> SFFYDRSTLSSVLQSTSDVSSKFTPSTAKNLQNSILLTPLPSDIVNNSVLPEQERWISFASPTTQKPPYKTKQDWNFIMFSPFTYYKCDLEVTLSKNDRETISSVVRYVPCGAPSDLSDQTMPQTPSLADTRDPHMWVVGQGTTNQISFVIPYTSPLSVLPSVWFNGFSNFDNSSRFGVAPNADFGRLLLQGQGTFSVHYRYKKMRVFCPRPTVFIPWP;> LLSLCKIPTFLGNLDSNKKRIPYFSATNSTPATPLVTYQVTLSCSCMANSMLAAVARNFNQYRGSLNYLFVFTGSAMTKGKFLISYTPPGAGEPKTLDQAMQATYAIWDLGLNSSYNFTVPFISPTHYRQTSYNTPTITSVDGWLTVWQLTPLTYPLGVPNDSHILTLVSGGDDFTLRMPVTFTKYVPQ;> SDRVSSDTAGNTATNTQSTVGRLFGFGQRHKGKHPASCADTATDKVLAAERYYTIKLASWTKTQESFDHIRVPLPHALAGENGGVFSSTLRRHYLCKCGWRIQVQCNASQFHAGSLLVFMAPEFDTSNHSTEVEPRADTAFKVDANWQKHAQILTGHAYVNTTTKVNVPLALNHQNFWQWTTYPHQILNLRTNTTCDLEVPYVNVCPTSSWTQHANWTLVIAVLTPLQYSQGSATTIEITASIQPVKPVFNGLRHTVV

Human Saffold virus 3 (SAFV-3) belongs to the species Theilovirus in the genus Cardiovirus of the family Picornaviridae. SAFVs cause diseases ranging from gastrointestinal disorders to meningitis. Cardioviruses have nonenveloped virions with an external diameter of about 30 nm. The major capsid proteins VP1 to VP3 form the capsid shell with pseudo-T=3 icosahedral symmetry whereas VP4 subunits are attached to the inner surface of the capsid.

The formation of SAFV-3 A particles can be induced by heating the virions to 42°C for 2 min. Here, we present a 10.6-Å resolution cryo-EM reconstruction of the SAFV-3 A particle and show that it is expanded 4% in diameter compared to the native virion. Capsids of SAFV-3 A particles have pores located approximately in the middle between the 5-fold and 3-fold icosahedral symmetry axes at the interface between two VP1 subunits related by a 5-fold symmetry axis and a VP3 subunit. The pores are circular in shape with a diameter of ∼15 Å. Models of the capsid protein subunits determined in the native SAFV-3 structure were fitted as rigid bodies into the native cryo-EM density map of the A particle. The formation of the pore is caused by shifts of the VP1 subunits toward the icosahedral 5-fold axis and of VP3 toward the icosahedral 3-fold axis relative to their positions in the native virus. Low values of density at the border of the pore indicate that the EF loop and C terminus of VP1 and CD, GH loops and C terminus of VP3, which are the located in the vicinity of the pore, are flexible. A difference map calculated by subtracting the electron density map of the SAFV-3 A particle from that of the native virion indicates that VP4 is missing from the A particle. SAFV-3 A particles do not contain pores at icosahedral 2-fold symmetry axes. The RNA does not form any contacts with the capsid of the A particle, unlike in the previously studied A particles of enteroviruses.>[2x]MAHHHHHHMVGLIWAQSTSGVIGRGGDIPWRVPEDLSHFKRITMGHTVVMG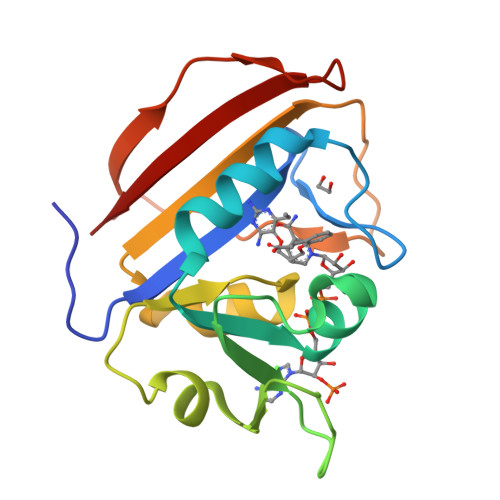RRTWDSLPASARPLPGRRNVVLSRQPGFVAEGAEVVGSLEDALTGPEDTWVIGGEQIYTLALPRAIRCEVTEVDVDLPRDDDDALAPPLDETWQGDVGEWQVSRSGLRYRFHSYYR> A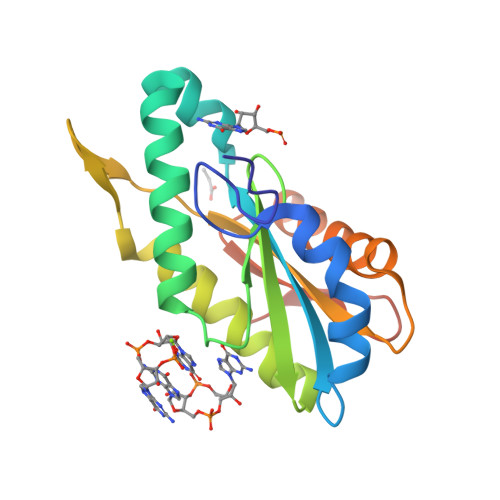IRSNMDVLTGLPGRRVLDESFDHQLRNAEPLNLYLMLLDIDRFKLVNDTYGHLIGDVVLRTLATYLASWTRDYETVYRYGGEEFIIIVKAANDEEACRAGVRICQLVDNHAITHSEGHINITVTAGVSRAFPEEPLDVVIGRADRAMYEGKQTGRNRCMFIDEQNVINRVLEHHHHHH>GTLTGERPPVFWLQGQGCTGCSVTLLNSVHPSIADVLLKVISLEFHPTVMAWEGEHAIEHMRKVAEKFKGKFFLVIEGSVPVEADGKYCIIGEANHHEISMVDALKEFGPNAAAVLAVGTCAAYGGIPAAEGSETGATAVSKFLGDNGIKTPVVNIPGCPPHPDWIVGTVVLALDAIKKNGLEGGLAEVVKVLDSDGRPTPFFGRNIHENCPYLDKYDEGVMSATFTDKVGCRYDLGCKGPMTMADCFERKWNGGVNWCVQNAVCIGCVEPDFPDGKSPFYQA[2x];>GATGRTTIAIDPVTRIEGHLKAEVVVENGKVVDARLSGGMYRGFETILRGRDPRDASQIVQRICGVCPTAHSTASVLALDEAFGAKVPNNGRITRNLIFGANYLQSHILHFYHLSAQDFVQGPDTAPFVPRFPKSDLRLSKELNKAGVDQYIEALEVRRICHEMVALFGGRMPHVQGQVVGGATEIPTKEKLVEYAARFKKVRDFVEQKYVPVVYTIGSKYKDMFKVGQGFKAALCVGAFPLDNSGKKHLFMPGVYAKGKDMPFDPSKIKEYVKYSWFAEETTGLNYKEGKTIPAPDKAGAYSFVKAPRYDGLS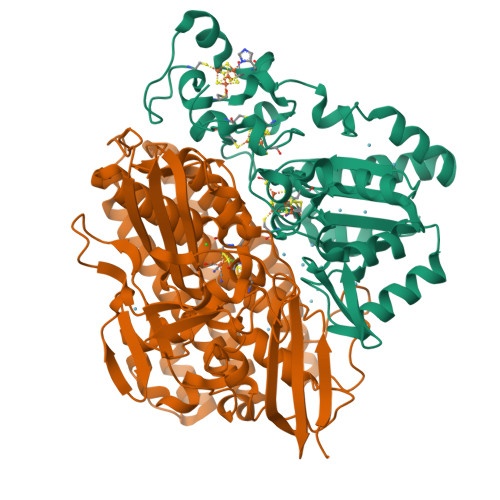LEVGPLARMWVNNPELSPVGKKLLKDLFGISAKKFRDLGEEAAFSLMGRHVARAEETYYMLGAIEGWLKEIKAGEDTVVMPAVPASAEGTGFTEAPRGSLLHYVKVKDSKIDNYQIVSASLWNCNPRDDMGQRGAVEEALIGIPVDDIQNPVNVARLIRAFDPULGCAVH[2x]Toll-like receptors (TLRs) play an important role in the innate immune response. Receptors belong to the type I of membrane proteins and contain the large extracellular ligand-binding domain, single-pass transmembrane domain, and globular intracellular Toll-interleukin receptor homology (TIR) domain. In particular, TLR1 is shown to form the heterodimers with TLR2, which are activated upon the binding of lipoteichoic acid or cysteine-containing lipopeptides. The overall fold of the resolved structure is typical for the TIR domains: five α-helices and a five-strand β-sheet.

We undertook several attempts to crystallize the TLR1-TIR/Zn complex. Similar to TLR1-TIR without Zn, crystals appeared in several months in P6422 and P6222 space groups, where the last one gave better diffraction. The best crystal diffracted to 1.9 Å and was used for the structure solution. All the crystals that were obtained provided the electron density with the Zn2+ ions absent and all cysteine residues in the oxidized state, similar to the structure of TLR1-TIR without Zn. We assume that the disulfide crosslinked conformation of TLR1-TIR is the only state of the protein capable of crystallization. In our hands, the protein was as well crystallized with the disulfide bonds, being formed in the presence of TCEP agent, whereas no disulfide bonds were observed in several weeks after the sample preparation for the soluble fraction of TLR1-TIR in solution under the similar conditions. It is noteworthy that crystal growth was essentially slow and took several months, and all the reducing agents have a limited lifetime. Thus, it is most likely that the protein crystallization started at a time point when no active TCEP was present in all the buffers, allowing the formation of cysteine bridges inevitably observed in crystallographic structures and necessary for the crystal packing.

> SNIPLEELQRNLQFHAFISYSGHDSFWVKNELLPNLEKEGMQICLHERNFVPGKSIVENIITCIEKSYKSIFVLSPNFVQSEWCHYELYFAHHNLFHEGSNSLILILLEPIPQYSIPSSYHKLKSLMARRTYLEWPKEKSKRGLFWANLRAAINIKLTEQAK> GHDRARTVQTALDLLNESGLDTLTMRRLAQAMDVQAGALYRYFAAKQDLLTAMAEHMVDGVADAAGATGDGDWSERTARLARALRAALLAHRDGARVFAGTHATGPNTLRFADGLVGVLREAGFG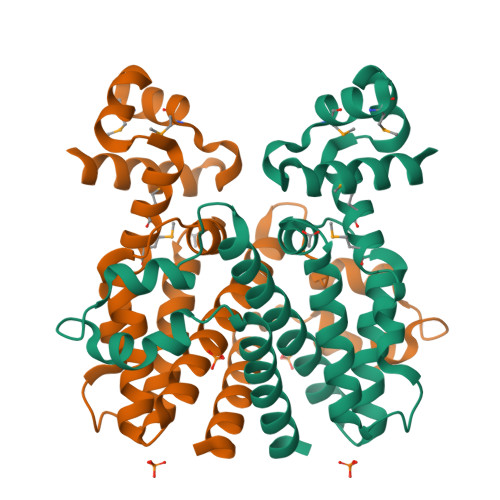DGDAARALYSVANFTVGHTLEEQAALTPGGGGPLDEATLREAVAAGTYPHLAATLPVLTSTDFTAHFEFGLRLLLDGLRAVRGS> MQNALKVGFWPAYSVSEFPPSKINSRLFTHLYYAFAELNAPTFEVRVPPGSEKTAEDFTPTVRRLNPSVKTLISIGGGGSEVRDNFAKLNSDASARQRFVKSSIALARRYGFHGLDLDYEYPEPQLEMENFVKLVSELTAAIREEARTSGKP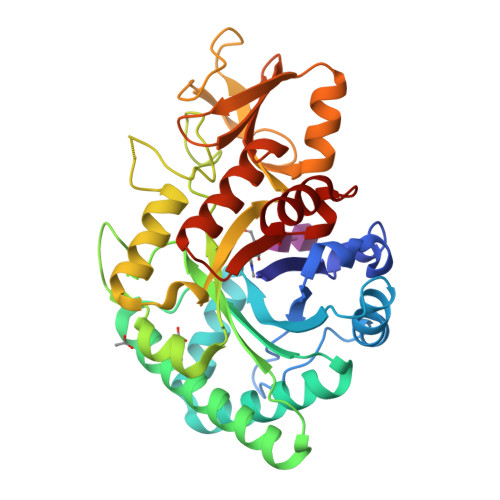RLLLTEAVYFHQKLFPWEVVTEYPVQFIAAGLDWVNVMAYDFHGSWENFTGAPAALRDPNSKFTASVGIESFLAAGMPPEKLVLGIPLFGRSWLLKNNNEVGIGAPAVGAGPVDGALSFSEIQNFIRGGAREVFDTTTVSAYAYKDNVWVGYDNQQSVALKVQYAKEKRLGGYFFWSVNQDIDAILPKIASDTWGG>[4x]MEKMD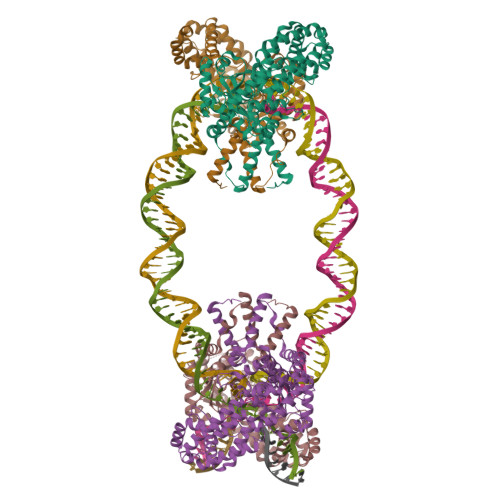NLEVKAKINQGLYKITPRHKGTSFIWNVLADIQKEDDTLVEGWVFCRKCEKVLKYTTRQTSNLCRHKCCASLKQSRELKTVSADCKKEAIEKCAQWVVRDCRPFSAVSGSGFIDMIKFFIKVGAEYGEHVNVEELLPSPITLSRKVTSDAKEKKALISREIKSAVEKDGASATIDLWTDNYIKRNFLGVTLHYHENNELRDLILGLKSLDFERSTAENIYKKLKAIFSQFNVEDLSSIKFVTDRGANVVKSLANNIRINCSSHLLSNVLENSFEETPELNMPILACKNIVKYFKKANLQHRLRSSLKSECPTRWNSTYTMLRSILDNWESVIQILSEAGETQRIVHINKSIIQTMVNILDGFERIFKELQTCSSPSLCFVVPSILKVKEICSPDVGDVADIAKLKVNIIKNVRIIWEENLSIWHYTAFFFYPPALHMQQEKVAQIKEFCLSKMEDLELINRMSSFNELSATQLNQSDSNSHNSIDLTSHSKDISTTSFFFPQLTQNNSREPPVCPSDEFEFYRKEIVILSEDFKVMEWWNLNSKKYPKLSKLALSLLSIPASSAASERTFSLAGNIITEKRNRIGQQTVDSLLFLNSFYKNFCKLDI The RNA chaperone protein Hfq, a member of the Lsm/Sm protein superfamily, is widespread in the bacterial kingdom, where it facilitates gene regulation by small noncoding RNAs (sRNAs) and other types of posttranscriptional control. The structure of the Hfq “core” region from several different bacterial species has now been solved, and in all cases a conserved hexameric ring structure has been observed. Appended to the core of Hfq is a short variable N-terminal extension (NTE) that is usually only four amino acids long and a longer variable C-terminal domain (CTD) that is predicted to be unstructured. The CTD of Hfq in E. coli has recently been proposed to autoinhibit RNA annealing activity, as acidic residues at the very C-terminal tip of the protein mimic the nucleic acid phosphodiester backbone to displace RNA from the rim.

We have solved the X-ray crystal structure of Cc Hfq to 2.15-Å resolution, including the structure of the entire length of the Hfq CTD. Purified full-length Cc Hfq was crystallized, and the structure was solved using the Ec Hfq core hexamer as a molecular replacement search model. Four Hfq hexamers could be modeled in the crystal asymmetric unit, packing in an unusual arrangement with the hexamers positioned orthogonal to one another to generate an “open square”. From the electron density maps, residues in the short CTD of Cc Hfq could be visualized for several protomers within the asymmetric unit, in some cases allowing for modeling of the entire length of the CTD with a high degree of confidence. On modeling the Cc Hfq CTD, it became apparent that these extensions pack against the CTD of neighboring hexamers in an antiparallel manner. The Cc Hfq CTDs that are not directly involved in contacting neighboring hexamers are partially disordered. From the structure of Cc Hfq, it is clear that the acidic tip residues (DADD; residues 78–82) pack against the positive rim residues of the proximal face (R18, K19, and K21), with few direct contacts to the arginine patch on the distal side of the rim (R49 and R50). Specifically, aspartates 81 and 82 are positioned to make electrostatic interactions with lysine 19 and arginine 18, respectively. Finally, glutamate 75 from within the CTD forms a hydrogen bond with arginine 49 and serine 39 on the neighboring protomer within the Hfq hexamer. These interactions agree with the proposed autoinhibitory mechanism in which acidic tip residues pack against conserved positive rim residues on the core of Hfq to compete with nucleic acid binding to the rim and disfavor spurious RNA annealing events. The well-ordered CTD–rim interactions observed in our structure suggest that the short Cc Hfq CTD may provide even stronger autoinhibition than the longer and more flexible Ec Hfq CTD.

>[24x]MSAEKKQNLQDTFLNSVRKSKTPLTIFLVNGVKLQGVVSWFDNFCVLLRRDGQSQLVYKHAISTIMPAQPVQLYEPSADADD>[2x]LTNLVAEPFAKLEQDFGGSIGVYAMDTGSGATVSYRAEERFPLCSSFKGFLAAAVLARSQQQAGLLDTPIRYGKNALVPWSPISEKYLTTGMTVAELSAAAVQYSDNAAANLLLKELGGPAGLTAFMRSIGDTTFRLDRWELELNSAIPGDARDTSSPRAVTESLQKLTLGSALAAPQRQQFVDWLKGNTTGNHRIRAAVPADWAVGDKT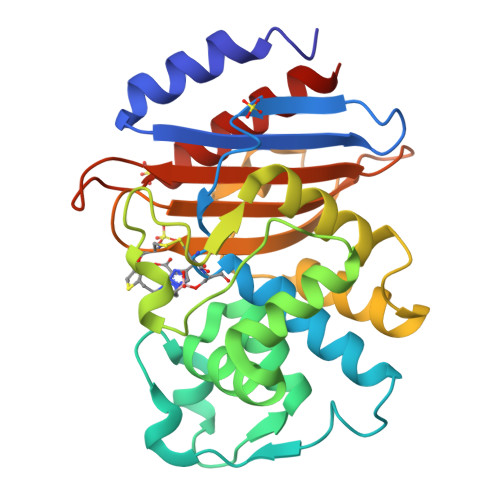GTCGVYGTANDYAVVWPTGRAPIVLAVYTRAPNKDDKHSEAVIAAAARLALEGLGVNGQ>[2x]MGSSHHHHHHSSGLVPRGSHVANTMASPNTPAPPNAAA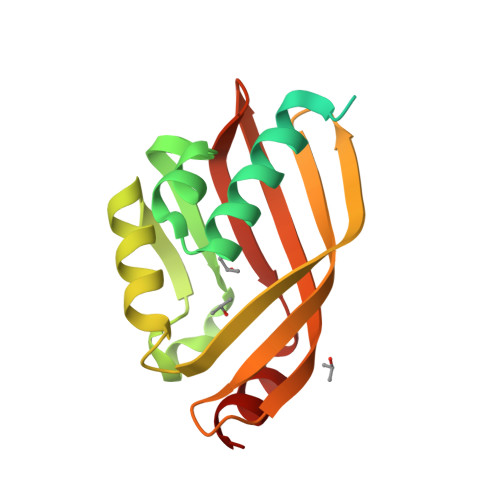SPNPSDSPNPSDSPNPPASPNIEAILASYAGFRDRDIEGILSGMHPDVEWVHPEGMGKYGLGGTKLGHAGIKEFLAHVPTVLGGMRLAPREFIEQGDRVVVFGTREVTSLRGTTATLDFVHSWTMRDGKATRMEDIFDTVAFHELIES>[8x]GHMSTLLINQPQYAWLKELGLREENEGVYNGSWGGRGEVITTYCPANNEPIARVRQASVADYEETVKKAREAWKIWADIPAPKRGEIVRQIGDALREKIQVLGSLVSLEMGKILVEGVGEVQEYVDICDYAVGLSRMIGGPILPSERSGHALIEQWNPVGLVGIITAFSFPVAVYGWNNAIAMICGNVCLWKGAPTTSLISVAVTKIIAKVLEDNKLPGAICSLTCGGADIGTAMAKDERVNLLSFTGSTQVGKQVGLMVQERFGRSLLELGGNNAIIAFEDADLSLVVPSALFAAVGTAGQRCTTARRLFIHESIHDEVVNRLKKAYAQIRVGNPWDPNVLYGPLHTKQAVSMFLGAVEEAKKEGGTVVYGGKVMDRPGNYVEPTIVTGLGHDASIAHTETFAPILYVFKFKNEEE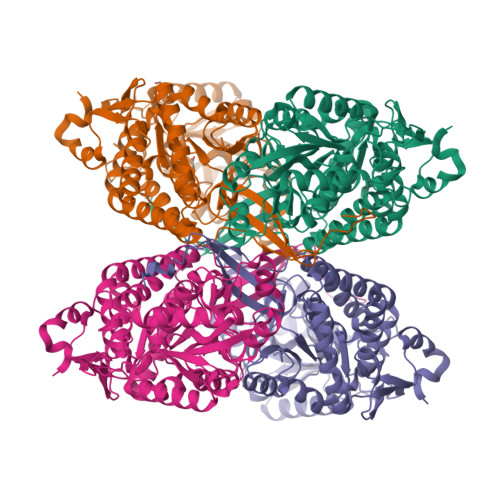VFAWNNEVKQGLSSSIFTKDLGRIFRWLGPKGSDCGIVNVNIPTSGAEIGGAFGGEKHTGGGRESGSDAWKQYMRRSTCTINYSKDLPLAQGIKFQ> SMKAEEARLEGKEYFTKSDWPNAVKAYTEMIKRAPEDARGYSNRAAALAKLMSFPEAIADCNKAIEKDPNFVRAYIRKATAQIAVKEYASALETLDAARTKDAEVNNGSSAREIDQLYYKAS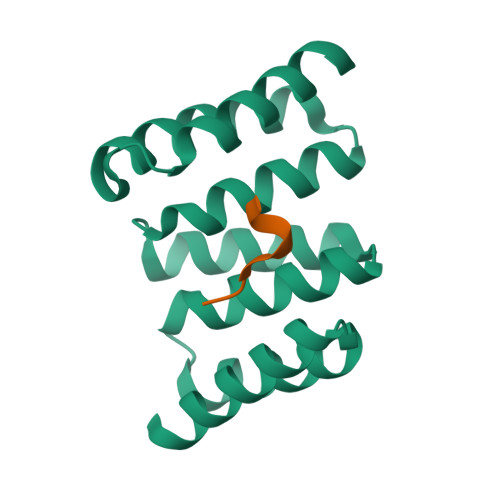QQRF;> PTVEEVD Nylon hydrolase (NylC) is one of the three enzymes responsible for the endo-type degradation of the by-products of nylon-6 manufacture (cyclic and linear oligomers of 6-aminohexanoate (Ahx) with a degree of polymerization greater than three) and various aliphatic nylons (e.g., nylon-6 and nylon-66). However, the post-translational autocleavage of the nascent polypeptide between Asn266 and Thr267 generates an active enzyme with an α subunit (27 kDa) and a β subunit (9 kDa). Based on the X-ray-crystallographic structure of NylCA, we reported that four αβ heterodimers (molecules A-D) form a doughnut-shaped quaternary structure. In addition, we proposed that the nucleophilic N-terminal residue Thr267 in the β subunit functions as a catalytic residue for either autocleavage (from precursor to active enzyme) or substrate hydrolysis.

To extensively analyze the effect of amino acid substitution at position 122, we constructed 10 new mutants in which Asp122 of NylCp2 was replaced with other amino acids by site-directed mutagenesis. The values of Tm (melting point of the heat denaturation) and ΔH (change in enthalpy for the global unfolding of proteins) were determined by regression analysis using nonlinear least-squares fitting of the CD melting curve. The Tm values increased in the order of Asp122 (wild-type NylCp2) < Leu < Gln < Asn < Arg < Lys < Val < Gly and ranged from 52.9 °C to 75.1 °C (type 1 mutation in Fig. 2). However, the D2 symmetry was partly altered by mutations at position 122. Plotting the protein stability (Tm value) estimated from the CD analyses against the distance between the two monomer molecules revealed that the protein stability exhibited an inverse correlation with the a2/a1 ratio (index of symmetry). In other words, the ratio changed from 0.979 to 1.197 from the wild-type (Asp122) to the mutant (Arg122, Lys122, Val122, and Gly122) enzyme, although this value should be equal to one for a perfectly symmetric structure. A clearer correlation was found between thermostability and the nearest distance between the side-chain atoms on helix α2 and helix α1. Notably, this distance decreased with an almost linear correlation with increasing thermostability in the wild-type and mutant enzymes.

>[2x]MNTTPVHALTDIDGGIAVDPAPRLAGPPVFGGPGNDAFDLAPVRSTGREMLRFDFPGVSIGAAHYEEGPTGATVIHIPAGARTAVDARGGAVGLSGGYDFNHAICLAGGAGYGLEAGAGVSVALLERLEHRTGFAELQLVSSAVIYDFSARSTAVYPDKALGRAALEFAVPGEFPQGRAGAGMSASAGKVDWDRTEITGQGAAFRRLGDVRILAVVVPNPVGVIVDRAGTVVRGNYDAQTGVRRHPVFDYQEAFAEQVPPVTEAGNTTISAIVTNVRMSPVELNQFAKQVHSSMHRGIQPFHTDMDGDTLFAVTTDEIDLPTTPGSSRGRLSVNATALGAIASEVMWDAVLEAGK>STGGVSPAATSAPLDWTTFRRVFLIDDAWRPLMEPELANPLTAHLLAEYNRRCQTEEVLPPREDVFSWTRYCTPDEVRVVIIGQDPYHHPGQAHGLAFSVRANVPPPPSLRNVLAAVKNCYPEARMSGHGCLEKWARDGVLLLNTTLTVKRGAAASHSRIGWDRFVGGVIRRLAARRPGLVFMLWGTHAQNAIRPDPRVHCVLKFSHPSPLSKVPFGTCQHFLVANRYLETRSISPIDWSV[2x];>[4x]VQNDFLDSYDVTMLL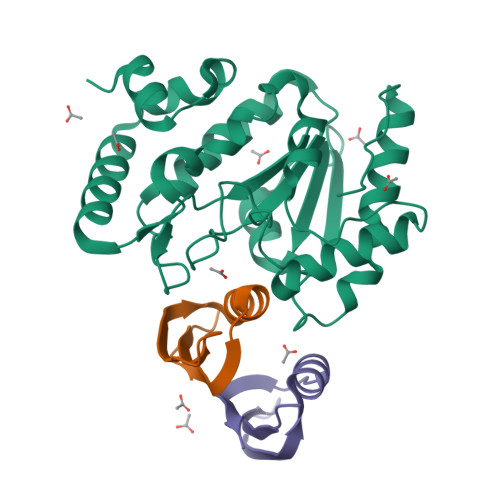QDDNGKQYYEYHKGLSLSDFEVLYGNTVDEIIKLRVDKIS3-(methylsulfonyl)-2-oxopropanoic acid | C4 H6 O5 S | 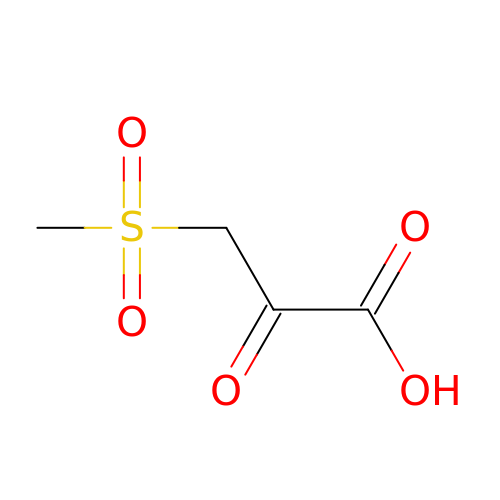KHOMRFGIBYBMCN-UHFFFAOYSA-N> ASPQRGRPRLNAARTTFVGDNGQPLRGPYTSTEWTAAAPYDQIARVKELGFNAVHLYAECFDPRYPAPGSKAPGYAVNEIDKIVERTRELGLYLVITIGNGANNGNHNAQWARDFWKFYAPRYAKETHVLYEIHNEPVAWGPPYSSSTANPPGAVDMEIDVYRIIRTYAPETPVLLFSYAVFGGKGGAAEALKDIRAFNKAVFGNENAVWTNEAVAFHGYAGWQETTIAVEELLKAGYPCFMTEYAGGAWGSGMGGLDVELTYELERLGVSWLTFQYIPPTGVSDDVTKPEYFSALVENSGLSWTPDYGNWPAARGVYGNGGLARETATWINNFLTGTTRIEAEDFDWGGNGVSYYDTDSVNVGGQYRPDEGVDIEKTSDTGGGYNVGWISEGEWLEYTIRVRNPGYYNLSLRVAGISGSRVQVSFGNQDKTGVWELPATGGFQTWTTATRQVFLGAGLQKLRINALSGGFNLNWIELSPISTGTIPDGTYKFLNRANGKTLQEVTGNNSIITADYKGITEQHWKIQHIGGGQYRISSAGRGWNWNWWMGFGTVGWWGTGSSTCFIISPTGDGYYRIVLVGDGTNLQISSGDPSKIEGKAFHGGANQQWAILPVSAPAFPTGLSAVLDSSGNTANLTWNAAPGANSYNVKRSTKSGGPYTTIATNITSTNYTDTGVATGTKYYYVVSAVSNGVETLNSAEAILQYPKLTGTVIGTQGSWNNIGNTIHKAFDGDLNTFFDGPTANGCWLGLDFGEGVRNVITQIKFCPRSGYEQRMIGGIFQGANKEDFSDAVTLFTITSLPGSGTLTSVDVDNPTGFRYVRYLSPDGSNGNIAELQFFGTPAGEENDDVHLGDILEHHHHHH

The GH5 arabinoxylanase (CtXyl5A) derived from Clostridium thermocellum displays an absolute requirement for xylans that contain Araf side chains. In this enzyme, the key specificity determinant is the Araf appended to O3 of the Xylp bound in the active site (−1 subsite). The dockerin domain recruits the enzyme into the cellulosome, a multienzyme plant cell wall degrading complex presented on the surface of C. thermocellum.

To explore further the role of the non-catalytic modules in CtXyl5A the crystal structure of CtXyl5A extending from CtGH5 to CtCBM62 was sought. Using this construct (CtXyl5A-D) the crystal structure of the arabinoxylanase was determined by molecular replacement to a resolution of 2.64 Å with Rwork and Rfree at 23.7% and 27.8%, respectively. The structure comprises a continuous polypeptide extending from Ala36 to Trp742 displaying four modules GH5-CBM6-CBM13-Fn3. Although there was some electron density for CtCBM62, it was not sufficient to confidently build the module. We postulate that the reason for the poor electron density is due to the CtCBM62 being mobile compared with the rest of the protein. In the structure of CtXyl5A-D, the four modules form a three-leaf clover-like structure. CtCBM13 acts as the central domain, which interacts with CtGH5, CtCBM6, and CtFn3 via 2, 5, and 4 hydrogen bonds, respectively, burying a surface area of ∼450, 350, and 500 Å2, respectively, to form a compact heterotetramer. The interactions between CtGH5 and the two CBMs, which are mediated by the tip of the loop between β-7 and α-7 (loop 7) of CtGH5, not only stabilize the trimodular clover-like structure but also make a contribution to catalytic function. Central to the interactions between the three modules is Trp285, which is intercalated between the two CBMs. Thus, any perturbation of the loop (through the removal of CtCBM13) is likely to influence the electrostatic and apolar environment of the catalytic apparatus, which could explain the reduction in activity associated with the deletion of CtCBM13.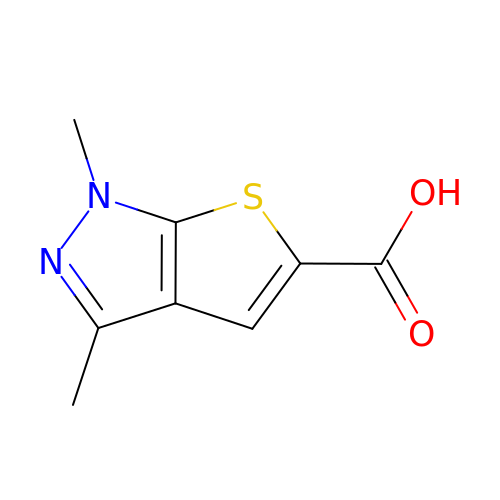1,3-dimethyl-1H-thieno[2,3-c]pyrazole-5-carboxylic acid | C8 H8 N2 O2 S | QRANSYHQSVJLHX-UHFFFAOYSA-N>MNALIVPQWPLPKGVAACSSTRIGGVSLSPYDSLNLGAHCGDNPEHVEENRKRLFAAGNLPSKPVWLEQVHGKNVLRLTGEPYASKRADASYSNTPGTVCAVMTADCLPVLFCNREGTEVAAAHAGWRGL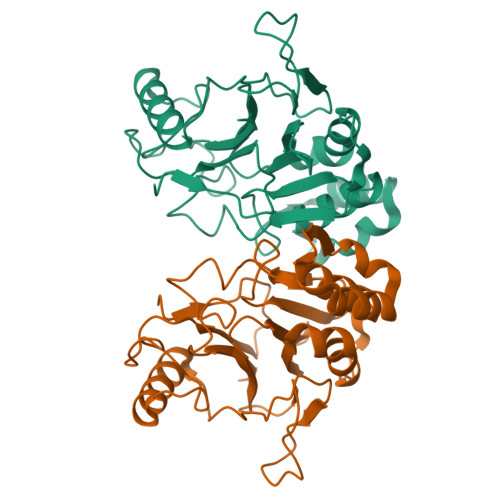CEGVLEETVTCFADKPENIIAWLGPAIGPAAFEVGPEVRDAFLAKDAQADSAFLPHGEKFLADIYQLARQRLANTGVEHVYGGDRCTFSESETFFSYRRDKTTGRMASFIWLI[2x]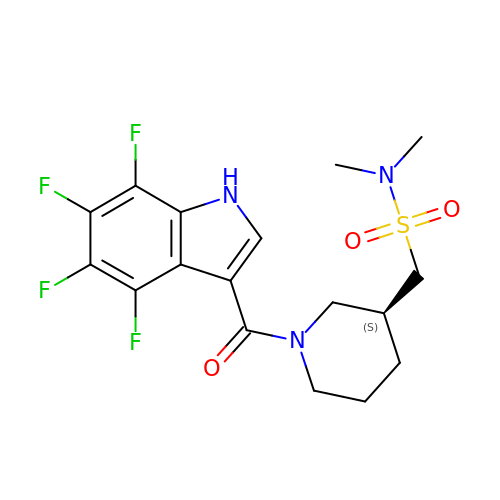~{N},~{N}-dimethyl-1-[(3~{S})-1-[[4,5,6,7-tetrakis(fluoranyl)-1~{H}-indol-3-yl]carbonyl]piperidin-3-yl]methanesulfonamide | C17 H19 F4 N3 O3 S | WWUFKLXXIIQYLV-VIFPVBQESA-N> MNSNNPDNNNSNNINNNNKDKDIAPNSDVQLATVYTKAKSYIPQIEQVYQGTNPNIQEAKLLGELLQVLAEVPKGTHLFCDPILEPISIFSLTIFSFNEEATATWLKNHFNPILSVCDKCILNFARGKCKMLQHFAIQRHVPHEHVAKFNDIVCQWRVEAVFPILRNISVNDNTGINITNEIETAMYECLCNPHMLRLNKQLKATFEAIFKFFYDTKHRLLDVTNPLSIKTFISGVIFCWCEGSKEENEWSRAFLKDLYSRNFHINLSNLTPDIIEEVYIHILFLQNPANWTEIVVSQFWSRLLPVFNLFDKDVFIEYFQVPKNVESLKKTFKFPLEPIFKMWYNHLSKSYHDKPLDFLLRGLTMFLNKFGSEFWSKIEPFTFHSILDIIFNRDSFPIKLIKIQDNPIVEHQTEVYFQLTGSVTDLLSWTLPFYHALSPSKRIQMVRKVSMAFLRIIANYPSLKSIPKACLMNSATALLRAVLTIKENERAM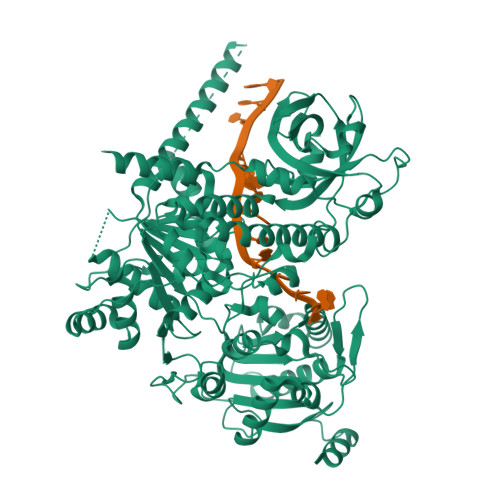LYKNDEFETVLLTKTDSRALLNNPLIQDIIIRSASNPNDFYPGLGAASASVATSTMMVLAECIDFDILLLCHRTFKLYSGKPISEIPISTNVLENVTNKIDLRSFHDGPLLAKQLLVSLKNINGLLIVPSNTAVAEAHNALNQKFLLLSTRLMEKFADILPGQLSKILADEDASQGFWSCIFSSDKHLYQAATNILYNTFDVEGRLEGILAILNSNLTVNLKNINVMLQRLINCEFYEPCPRAVRVLMDVVSAFVDPISGVFANFQTLKSQNTEKEFLKFWESCWLFLDTIYKFTLKWASKYDYSELENFTKDTLDLSRSLVDSFREFSDILHDQTKNLLLNVLETFKNMLYWLRLSDEVLLESCVRLIISTSDLAHEKHVKVDDSLVEMMAKYASKAKRFSNKLTEQQASEILQKAKIFNKALTEEVATEAENYRKEKELSRLGKVIDLTDSVPASPSLSPSLSSTIASSSAESRADYLQRKALSSSITGRPRVAQPKITSFGTFQSSANAKLHRTKPVKPLSKMELARMQLLNNRVVHPPSAPAFHTKSRGLSNKNDDSSSEESDNDIESARELFAIAKAKGKGIQTVDINGKVVKRQTAAELAKQELEHMRKRLNVDMNPLYEIILQWDYTRNSEYPDDEPIGNYSDVKDFFNSPADYQKVMKPLLLLESWQGLCSSRDREDYKPFSIIVGNRTAVSDFYDVYASVAKQVIQDCGISESDLIVMAYLPDFRPDKRLSSDDFKKAQHTCLAKVRTLKNTKGGNVDVTLRIHRNHSFSKFLTLRSEIYCVKVMQMTTIEREYSTLEGLEYYDLVGQILQAKPSPPVNVDAAEIETVKKSYKLNTSQAEAIVNSVSKEGFSLIQGPPGTGKTKTILGIIGYFLSTKNASSSNVIKVPLEKNSSNTEQLLKKQKILICAPSNAAVDEICLRLKSGVYDKQGHQFKPQLVRVGRSDVVNVAIKDLTLEELVDKRIGERNYEIRTDPELERKFNNAVTKRRELRGKLDSESGNPESPMSTEDISKLQLKIRELSKIINELGRDRDEMREKNSVNYRNRDLDRRNAQAHILAVSDIICSTLSGSAHDVLATMGIKFDTVIIDEACQCTELSSIIPLRYGGKRCIMVGDPNQLPPTVLSGAASNFKYNQSLFVRMEKNSSPYLLDVQYRMHPSISKFPSSEFYQGRLKDGPGMDILNKRPWHQLEPLAPYKFFDIISGRQEQNAKTMSYTNMEEIRVAIELVDYLFRKFDNKIDFTGKIGIISPYREQMQKMRKEFARYFGGMINKSIDFNTIDGFQGQEKEIILISCVRADDTKSSVGFLKDFRRMNVALTRAKTSIWVLGHQRSLAKSKLWRDLIEDAKDRSCLAYACSGFLDPRNNRAQSILRKFNVPVPSEQEDDYKLPMEYITQGPDEVKSNKDTKKRRVVDEGEEADKAVKKKKKEKKKEKKKSKADDKKKNNKKAESPSTSSGTKKKSSIFGGMSVPSAVVPKTFPDVDSNKKAAAVVGKKKNNKHVCFSDDVSFIPRNDEPEIKVTRSLSSVLKEKQLGLKETRTISPPEISNNEDDDDEDDYTPSISDSSLMKSEANGRNNRVASHNQNFSASIYDDPQVSQAKQTQVPAAITKHRSSNSVLSGGSSRILTASDYGEPNQNGQNGANRTLSQHVGNANQYSTAPVGTGELHETLPAHPQDSYPAEAEDPYDLNPHPQPQSSAFKGPGSGPTGTRNSSRRNASSSPFIPKKRKPRS> MEIKKGLEDVYVKETEITYIDGELGRLYYRGYSIYDLAEFSNFEEVSYLILYGKLPNREELNWFQEKLREERYLPDFIIKFLREVRKDAQPMDILRTAVSLLGIEDSKNDERTDIKGIKLISKFPTIVANYARLRKGLDIIEPDPKLSHSENFLYMLYGDRPNEIKSKAMDVTLILHIDHEMNASTFASLVVASTFSDLYSSIVAGISALKGPLHGGANYEALKMFKEIGSPEKVNDYILNRLSNKQRIMGFGHRVYKTYDPRARILKQYAKLLAEKEGGEIYTLYQIAEKVEEIGIKYLGPKGIYPNVDFFSSIVFYSLGFEPDFFPAVFASARVVGWVAHIMEYIKDNKIIRP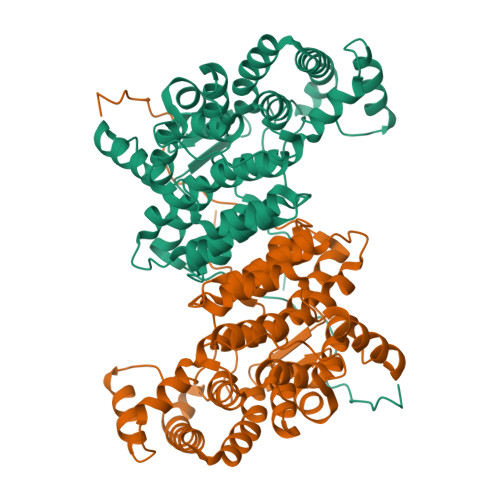KAYYKGEIGKKYIPIDSR>[4x]SAKILAIDTATENCSVALLVNDQVISRSEVAPRDHTKKVLPMVDEVLKEAGLTLQDLDALAFGRGPGSFTGVRIGIGIAQGLAFGAELPMIGVSTLAAMA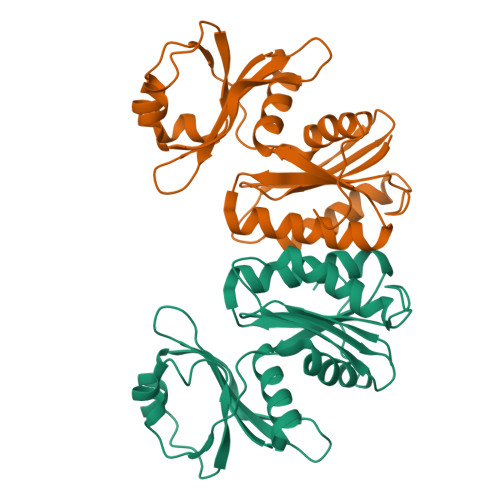QASYRLHGATDVAVAIDARMSEVYWARYSRQENGEWIGVDEECVIPPARLAEEAQADSKTWTTAGTGWSAYQEELAGLPFNTADSEVLYPDSQDIVILAKQELEKGNTVPVEE> GIDPFTHMATFISVQLKKTSEVDLAKPLVKFIQQTYPSGGEEQAQYCRAAEELSKLRRAAVGRPLDKHEGALETLLRYYDQICSIEPKFPFSENQICLTFTWKDAFDKGSLFGGSVKLALASLGYEKSCVLFNCAALASQIAAEQNLDNDEGLKIAAKHYQFASGAFLHIKETVLSALSREPTVDISPDTVGTLSLIMLAQAQEVFFLKATRDKMKDAIIAKLANQAADYFGDAFKQCQYKDTLPKEVFPVLAAKHCIMQANAEYHQSILAKQQYYFGEEIARLQHAAELIKTVASRYDEYVNVKDFSDKINRALAAAKKDNDFIYHDRVPDLKDLDPIGKATLVKSTPVNVPISQKFTDLFEKMVPVSVQQSLAAYNQRKADLVNRSIAQMREATTLANGVLASLNLPAAIEDVSGDTVPQSILTKSRSVIEQGGIQTVDQLIKELPELLQRNREILDESLRLLDEEEATDNDLRAKFKERWQRTPSNELYKPLRAEGTNFRTVLDKAVQADGQVKECYQSHRDTIVLLCKPEPELNAAIPSANPAKTMQGSEVVNVLKSLLSNLD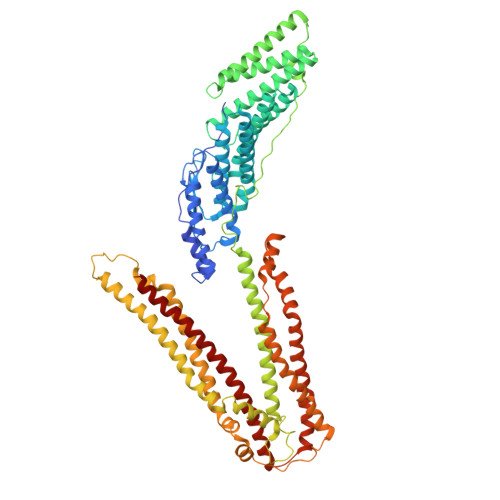EVKKEREGLENDLKSVNFDMTSKFLTALAQDGVINEEALSVTELDRVYGGLTTKVQESLKKQEGLLKNIQVSHQEFSKMKQSNNEANLREEVLKNLATAYDNFVELVANLKEGTKFYNELTEILVRFQNKCSDIVFAR In eukaryotes, the ubiquitin‐related modifier 1 (Urm1) pathway is responsible for the synthesis of 2‐thiolated wobble uridine (U34). Uba4 is a two‐domain protein containing an adenylation domain (AD) and a rhodanese‐like domain (RHD), which are both essential for the dual function of Uba4 in sulfur transfer and ubiquitin‐like conjugation (Furukawa et al, 2000; Huang et al, 2008; Schmitz et al, 2008; Leidel et al, 2009; Noma et al, 2009). Uba4 activates the C‐terminus of Urm1 via an ATP‐dependent adenylation step, receives mobilized sulfur from the Nfs1/Tum1‐relay system by its RHD, and subsequently forms thiocarboxylated Urm1 (Urm1‐COSH; Leidel et al, 2009; Noma et al, 2009). We heterologously expressed and purified Uba4 from Chaetomium thermophilum (CtUba4), a thermophilic fungus harboring highly stable proteins, well‐suited for X‐ray crystallography and other in vitro approaches (Bock et al, 2014).

Interestingly, the structure reveals a homo‐dimeric complex of two protein units with an asymmetric positioning of the ADs and RHDs, which themselves form individual dimers. While the ADs and RHDs individually form C2‐symmetrical dimers, the structure is asymmetric since the two 2‐fold axes do not coincide. The individual ADs are formed by a continuous sheet of eight β‐strands surrounded by eight α‐helices and are highly similar to both MoeB, the prokaryotic ancestor of Uba4, and to ADs of UBL E1 enzymes (Cappadocia & Lima, 2018; Lake et al, 2001; Olsen et al, 2010). Like the AD, the RHD forms a dimer mediated by hydrogen bonds between active‐site loop residues Arg398, Arg399, and Glu405 occluding the active cysteines (Fig EV1B), which suggests that the RHDs are inhibited in the apo form of Uba4. Noteworthy, the RHD dimer mainly interacts with only one AD. One Uba4 dimer harbors two nucleotide‐binding sites, formed by conserved residues of both ADs (Gly45, Arg77, Lys90, Asp134 of one subunit and Arg18 of the second subunit) implying that AD homodimerization is essential for the adenylation of Urm1 (Fig EV2A). Although Uba4 was crystallized in the absence of nucleotides, the highly conserved binding pocket enabled us to model an AMP molecule into the structure with high confidence. However, the function of this linker is undefined. We found that in one of the two Uba4 molecules, almost the entire linker adopts a stable conformation with a well‐defined electron density (Figs 2B and EV2B), while this is not the case for the second Uba4 molecule in the dimer. The structured linker closely interacts with the AD, and its residues, in particular Asn307 and Met308, are in close proximity to the ATP‐binding pocket, coinciding with the expected localization of the C‐terminus of Urm1 when bound to Uba4.

> STQKSLSKEEIERYSRQMIVPGMGKEGQLRLMNAKVLIIGAGGLGCPAAQYLAGAGVGTIGIVDGDSVETSNLHRQVAHATKRVGMLKVDSLITHLIEINPLPVYVPYRFDLTPQNAAQIIKPWDVILDCTDNPATRYLISDVCVLLGKPLVSAASVQKSGQLIVLNCPPTPQGVVNKKAAPCYRCCFKKPPPPSAQTSCGEAGIMGPVVGMMGVAQAGEAIKILVSQLHMPPKEGEEVSPEKNLVQPTLLIYTYDLNSAIGPYSFRALKMGGRKKDCFACGENSTLTLDGIKSGNPNYVQFCGNMTQSTNLAPEDRITATAYNEKRRNGELGEHILLDTREKEHFSFGSIPGAVNVPFSKFLVKASSIKREGNSPAELLPMQPASDEAPIVVVCRRGQDSQEVVEKLKELGLDNGGKRKIMDIVGGMKAWRDEVDPDFPFI;> GSTQKSLSKEEIERYSRQMIVPGMGKEGQLRLMNAKVLIIGAGGLGCPAAQYLAGAGVGTIGIVDGDSVETSNLHRQVAHATKRVGMLKVDSLITHLIEINPLPVYVPYRFDLTPQNAAQIIKPWDVILDCTDNPATRYLISDVCVLLGKPLVSAASVQKSGQLIVLNCPPTPQGVVNKKAAPCYRCCFKKPPPPSAQTSCGEAGIMGPVVGMMGVAQAGEAIKILVSQLHMPPKEGEEVSPEKNLVQPTLLIYTYDLNSAIGPYSFRALKMGGRKKDCFACGENSTLTLDGIKSGNPNYVQF;> DRITATAYNEKRRNGELGEHILLDTREKEHFSFGSIPGAVNVPFSKFLVKASSIKREGNSPAELLPMQPASDEAPIVVVCRRGQDSQEVVEKLKELGLDNGGKRKIMDIVGGMKAWRDEVDPDFPFI>[2x]SNANVGVFVLMHGDSTASSMLKTAQELLGTSIGTAMNMPLTMEVQTMYEQLRNQVITQKESLNNGILLLTDMGSLNS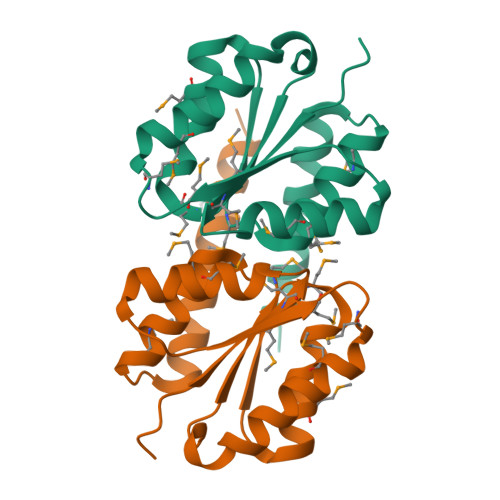FGNMLFEETGIRTKAITMTSTMIVLEAIRMASVGRSLEDIYQNIQLSFESVVREQFRSSLQK>[8x]MTPR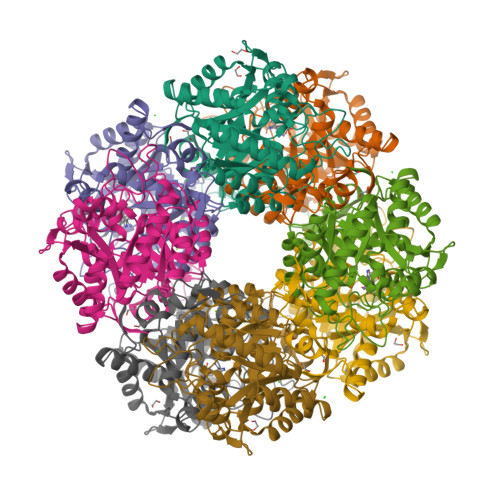GPLDNNNYGEVWLPIQARPRRNRKNRAVRQLVQENLVKPSSLIYPLFVHDEETSVPIPSMPGQSRLSMEDLLKEVGEARSYGIKAFMLFPKVDDELKSVMAEESYNPDGLLPRAIMALKEAFPDVLLLADVALDPYSSMGHDGVVDEQSGKIVNDLTVHQLCKQAITLARAGADMVCPSDMMDGRVSAIRESLDMEGCTDTSILAYSCKYASSFYGPFRDALDSHMVGGTDKKTYQMDPSNSREAEREAEADASEGADMLMVKPGLPYLDVLAKIREKSKLPMVAYHVSGEYAMLKAAAEKGYISEKDTVLEVLKSFRRAGADAVATYYAKEAAKWMVEDMKGTQKFTEPCY The savanna soil yeast Blastobotrys mokoenaii displays superior growth on xylan thanks to an efficient secreted glycoside hydrolase family 11 (GH11) xylanase; solving its crystal structure revealed a high similarity to xylanases from filamentous fungi. Xylan degradation requires an arsenal of CAZymes such as carbohydrate esterases (CEs) and glycoside hydrolases (GHs), with the most common xylan backbone-cleaving endo-β-1,4-xylanases being found in glycoside hydrolase family 10 (GH10), GH11, and GH30 (7, 8). Endo-β-1,4-xylanases are the main enzymes responsible for xylan depolymerization, supported by β-xylosidases. In this study, we characterized the xylanolytic strategies of three phylogenetically diverse yeasts with different CAZyme profiles: Blastobotrys mokoenaii (phylogenetically in the Trichomonascaceae clade; isolated from savanna soil), which possesses a GH11 and a GH30_7 xylanase, Scheffersomyces lignosus (CUG-Ser1 clade; isolated from the gut of wood-boring insects), which possesses a GH10 xylanase, and Wickerhamomyces canadensis (Phaffomycetaceae clade; isolated from Canadian red pine), which lacks any obvious endo-β-1,4-xylanases.

We successfully crystallized and solved the structure of BmXyn11A extending to 1.55-Å resolution, by molecular replacement using an AlphaFold2-predicted structure of BmXyn11A as the search model. The structure of the P. pastoris-expressed BmXyn11A is the first GH11 structure from a budding yeast. The overall structure adopted the expected GH11 β-jelly roll fold, and the asymmetric unit contained five protein molecules. Comparisons with previously solved GH11 members from bacteria and fungi show high conservation, even among kingdoms, with Cα-root mean square deviation (RMSD) values of <0.6 Å to BmXyn11A, which could suggest either retention of this enzyme in B. mokoenaii after the split between yeast and filamentous fungi or possibly a recent horizontal gene transfer event. BmXyn11A had the highest specific activity of the recombinant enzymes on xylan (4,350 U · mg−1), nearly 4-fold higher on beechwood GX than on the closely related GH11 XynB from Aspergillus niger An76 (1,146 U · mg−1). BmXyn11A reached near-maximum xylan hydrolysis levels after only 15 min, releasing mainly smaller XOs (xylose, X1; xylobiose, X2; and xylotriose, X3). The differences in XO distributions between BmXyn11A and SlXyn10A from GX correspond to previous studies, where GH11 xylanases require three unsubstituted xylose units for attack on the xylan backbone, while GH10 xylanases can accommodate more branched xylans. Secreted enzymes such as the GH11 xylanase from B. mokoenaii produce XOs in the extracellular environment, which could also benefit neighboring cells from other species and enable cross-feeding behavior. B. mokoenaii is the standout species thanks to its secreted powerful BmXyn11A, which likely facilitates the rapid growth on xylan.

>[5x]MKLSNAITAICAAAVLAAPLEEEEVAKRSVTPSSTGTNNGYYYSFWSDGGGDVTYTNGNGGSYSVEWTNCGNFVGGKGWNPGAAREINFSGSFNPSGNGYLSVYGWTTNPLVEYYIVESYGDYNPGTAGTFLGTVDSDGSTYDIYKAVRTNAPSIEGTATFDQYWSIRRNHRTSGTVNTGNHFNAWAQHGLQLGTHNYQIVATEGYQSSGSSSITVSVDHHHHHH>GSNVNKIYIENHDLMSKVPVIEASKESTRDDWAALTVVADLDDIEGQELVYYALRFRKSNDGVRLDIVHNPKDTSRSPSVLAQRLKSREDKLLDFTRFLDLETALETGEFEPDVAYDASLANFLASSNMKAGDNFVILN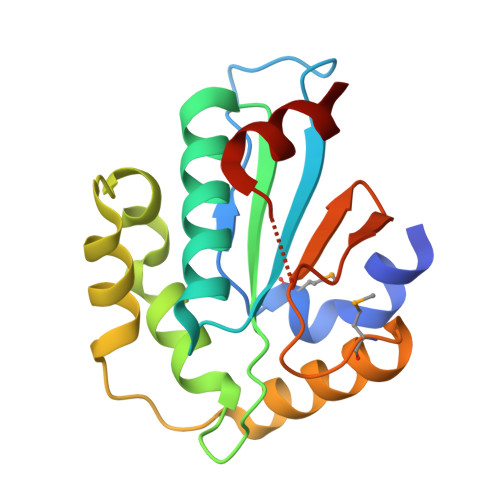GRVLGPITSADDFKKEDFEVFLQA[6x]3-(3-methylsulfonylphenyl)benzoic acid | C14 H12 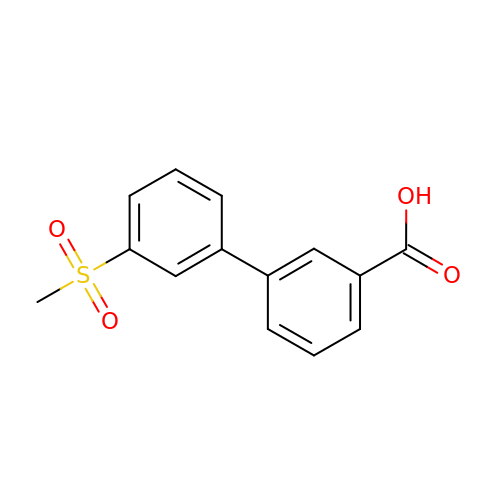O4 S | CRFKLEDBWMGUED-UHFFFAOYSA-N>MEKKKVAEWLAQGSIAVPKLLLGHYKQLGL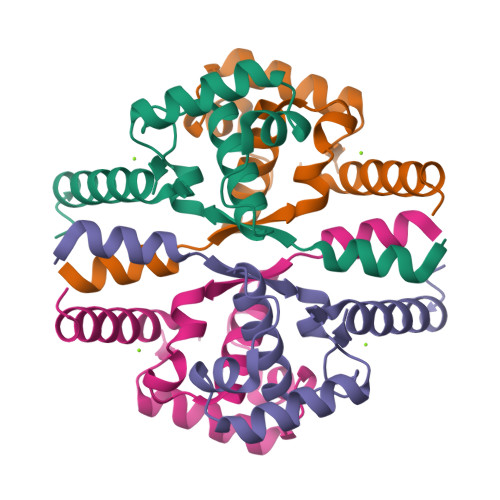GEGELVLLLHMQSFFEEGVLFPTPAELAERMTVSAAECMEMVRRLLQKGMIAIEEHTDEQGIRNEKYTLEPLWEKLVHHLYTQAAQQGELGRQEEEES[4x]>MLAVLEIGIIENVQRADLNVLEEALSYKVLMEKFERTQENIAQT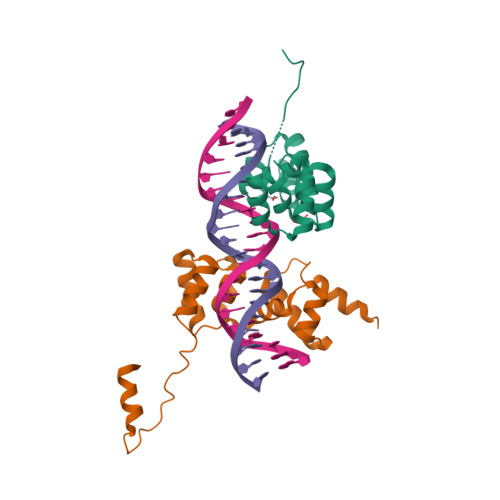IGKSRSHVANTMRLLALPDEVQSYLVSGELTAGHARAIAAAADPVALAKQIIEGGLSVRETEALARKAPNLSAGKSKGGRPPRVKDKLAAALEHHHHHH[2x]>[10x]DYKDDDK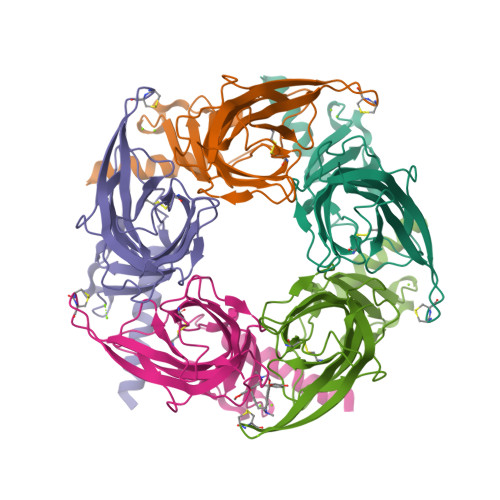LHSQANLMRLKSDLFNRSPMYPGPTKDDPLTVTLGFTLQDIVKADSSTNEVDLVYYEQQRWKLNSLMWDPNEYGNITDFRTSAADIWTPDITAYSSTRPVQVLSPQIAVVTHDGSVMFIPAQRLSFMCDPTGVDSEEGATCAVKFGSWVYSGFEIDLKTDTDQVDLSSYYASSKYEILSATQTRQVQHYSCCPEPYIDVNLVVKFRERRAGNGFFRNLFD> MGSSHHHHHHSSGENLYFQGSHMTATATSAKAAAPACPRFDDPVHAAADPRVDVERITPDPVWRTTCGTLYRSDSRGPAVVFEQGFLPKDVIDGQYDIESYVLVNQPSPYVATTYDHDLYKTWYKSGYNYYIDAPGGVDVNKTIGDRHKWADQVEVAFPGGIRTEFVIGVCPVDKKTRTEKMSECVGNPHYEPWH

S. scabies produces a 200-residue, 22-kDa protein that is a single-domain enzyme called Scabin. Scabin has been cloned, expressed, and purified, and shown to harbor dual enzymatic activities (GH and ADP-ribosyltransferase). Scabin targets DNA as a substrate for ADP-ribose modification; it also shows enzyme specificity towards genomic DNA from Solanum tuberosum tubers. Scabin shares nearly 40% sequence identity with the Pierisin family of mARTs.

Scabin has some common catalytic features with other members of the mART toxin family. This includes the key Arg (Arg77), which is important for NAD+ binding to the active site; the Ser-Thr-Thr motif (Ser117-Thr118-Thr119), which comprises the scaffold of the NAD+ binding site; and the hallmark catalytic Gln-X-Glu motif (Gln158-X-Glu160). Other residues that were studied included two NAD+-only interacting residues, such as Ser117 found in the STT(S) NAD+ binding motif and Glu160 in the Q-X-E motif. The S-T-S/T motif is known for its role in binding and positioning the NAD+ substrate in CT-like mART toxins. The rest of the Scabin variants showed either a WT-like crystal structure or similar CD spectra to the WT in solution. All the structures were of high quality, ranging from 1.5 to 1.75 Å.> GSIQQATTGVSQETSENPGDKTIVPATLPQLTPTLVSLLEVIEPEVLYAGYDSSVPDSTWRIMTTLNMLGGRQVIAAVKWAKAIPGFRNLHLDDQMTLLQYSWMSLMAFALGWRSYRQSSANLLCFAPDLIINEQRMTLPDMYDQCKHMLYVSSELHRLQVSYEEYLCMKTLLLLSSVPKDGLKSQELFDEIRMTYIKELGKAIVKREGNSSQNWQRFYQLTKLLDSMHEVVENLLNYCFQTFLDKTMSIEFPEMLA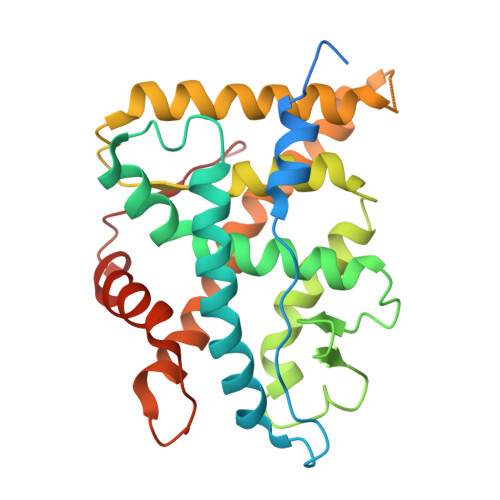EIITNQIPKYSNGNIKKLLFHQK> NLRGGAFVSNTQITMADKQKKFINEIQEGDLVRSYSITD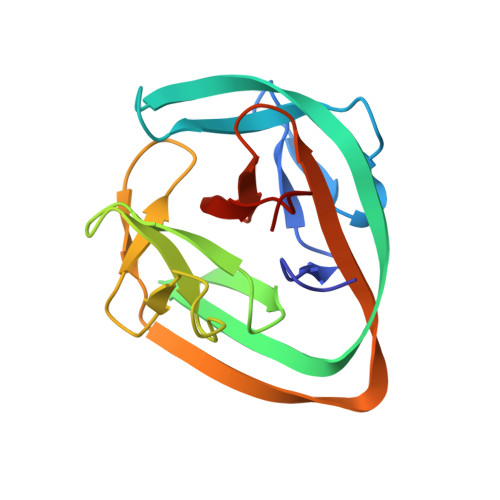ETFQQNAVTSIVKHEADQLCQINFGKQHVVCTVNHRFYDPESKLWKSVCPHPGSGISFLKKYDYLLSEEGEKLQITEIKTFTTKQPVFIYHIQVENNHNFFANGVLAHAMQVSI> GKV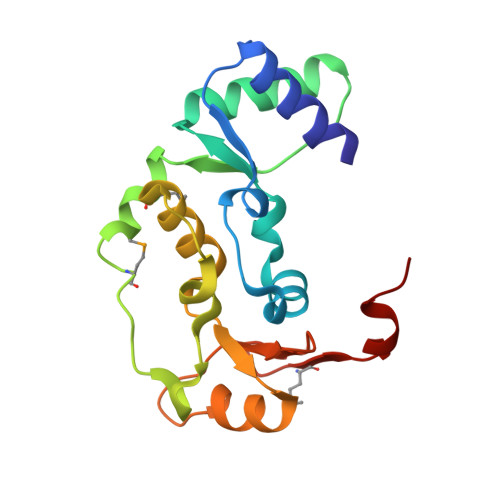LDAIIQEKKSGRIPGIYGRLGDLGAIDEKYDIAISSCCHALDYIVVDSIDTAQECVNFLKKHNIGIATFIGLDKMTVWAKKMSKIQTPENTPRLFDLVKVKNEEIRQAFYFALRDTLVANNLDQATRVAYQRDRRWRVVTLQGQIIEQSGTMSGGLEHHHHHH>[8x]MTTYGFLGLGIMGGPMAANLVRAGFDVTVWNRNPAKCAPLVALGARQASSPAEVCAACDITIAMLADPAAAREVCFGANGVLEGIGGGRGYIDMSTVDDETSTAIGAAVTARGGRFLEAPVSGTKKPA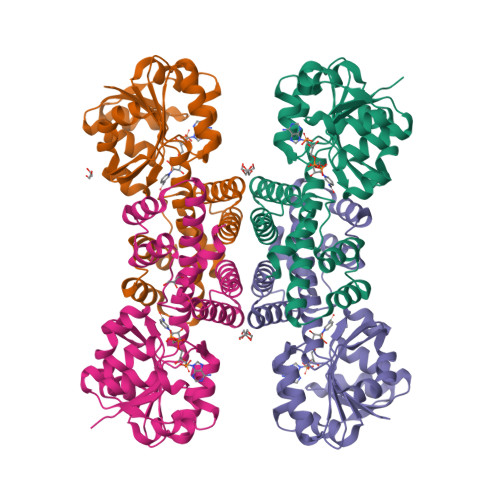EDGTLIILAAGDQSLFTDAGPAFAALGKKCLHLGEVGQGARMKLVVNMIMGQMMTALGEGMALGRNCGLDGGQLLEVLDAGAMANPMFKGKGQMLLSGEFPTSFPLKHMQKDLRLAVELGDRLGQPLHGAATANESFKRARAAGHADEDFAAVFRVLEA3-oxo-N-[(3S)-2-oxotetrahydrofuran-3-yl]hexanamide 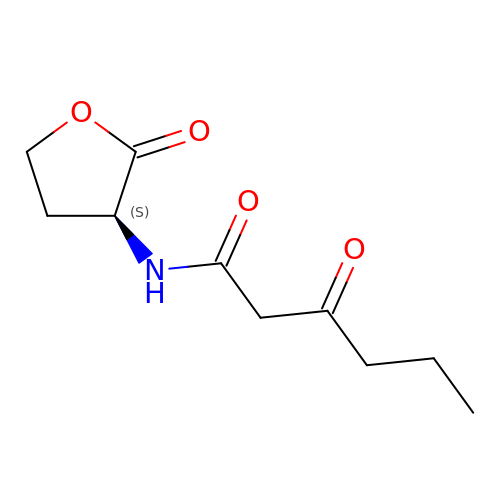| C10 H15 N O4 | YRYOXRMDHALAFL-QMMMGPOBSA-N>[14x]MNSSFPYFISPEQAMRERSELARKG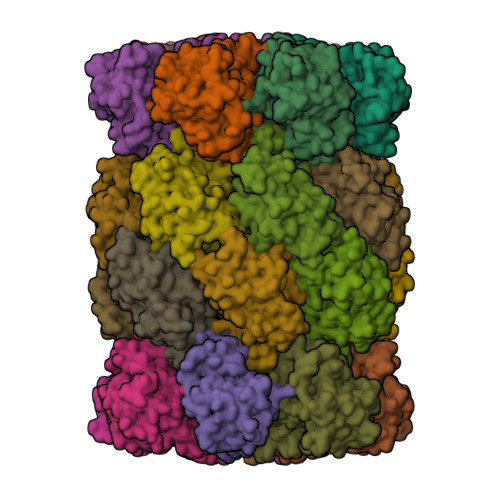IARAKSVVALAYAGGVLFVAENPSRSLQKISELYDRVGFAAAGKFNEFDNLRRGGIQFADTRGYAYDRRDVTGRQLANVYAQTLGTIFTEQAKPYEVELCVAEVAHYGETKRPELYRITYDGSIADEPHFVVMGGTTEPIANALKESYAENASLTDALRIAVAALRAGSADTSGGDQPTLGVASLEVAVLDANRPRRAFRRITGSALQALLVDQESPQSDGESSG;>[14x]TTIVALKYPGGVVMAGDRRSTQGNMISGRDVRKVYITDDYTATGIAGTAAVAVEFARLYAVELEHYEKLEGVPLTFAGKINRLAIMVRGNLAAAMQGLLALPLLAGYDIHASDPQSAGRIVSFDAAGGWNIEEEGYQAVGSGSLFAKSSMKKLYSQVTDGDSGLRVAVEALYDAADDDSATGGPDLVRGIFPTAVIIDADGAVDVPESRIAELARAIIESRSGADTFGSDGGEKHHHHHH> GGSPVSIKVQVPNMQDKTEWKLNGQVLVFTLPLTDQVSVIKVKIHEATGMPAGKQKLQYEGIFIKDSNSLAYYNMANGAVIHLALKER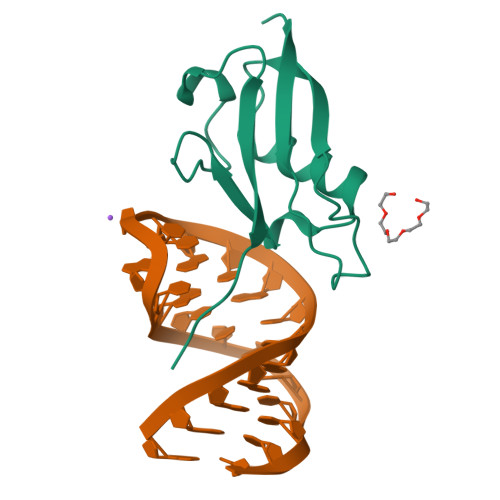GGRKK>[5x]MSSEQLHEPAELLSEETKNMHRALVTLIEELEAVDWYQQRADACSEPGLHDVLIHNKNEEVEHAMMTLEWIRRRSPVFDAHMRTYLFTERPILELEEEDTGSSSSVAASPTSAPSHGSLGIGSLRQEGKED;>[5x]MDLLKRHLAPIVPDAWSAIDEEAKEIFQGHLAGRKLVDFRGPFGWEY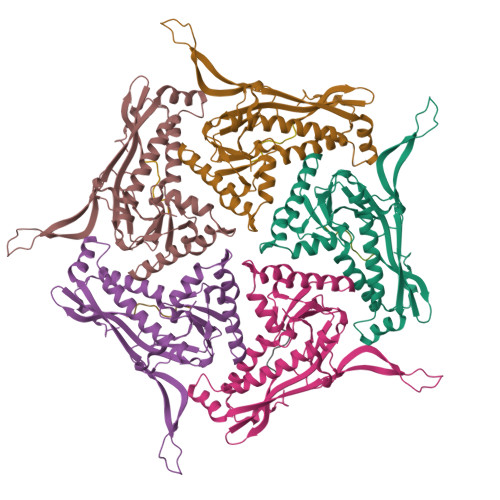AAVNTGELRPIDDTPEDVDMKLRQVQPLAEVRVPFTLDVTELDSVARGATNPDLDDVARAAERMVEAEDSAIFHGWAQAGIKGIVDSTPHEALAVASVSDFPRAVLSAADTLRKAGVTGPYALVLGPKAYDDLFAATQDGYPVAKQVQRLVVDGPLVRANALAGALVMSMRGGDYELTVGQDLSIGYAFHDRSKVELFVAESFTFRVLEPGAAVHLRYA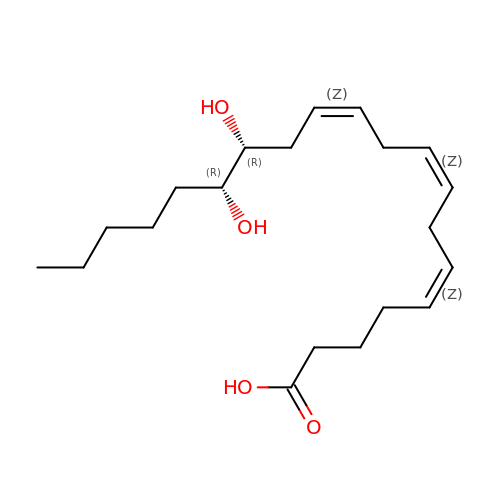(5~{Z},11~{Z},14~{R},15~{R})-14,15-bis(oxidanyl)icosa-5,8,11-trienoic acid | C20 H34 O4 | SYAWGTIVOGUZMM-JHIAIUNDSA-N>[2x]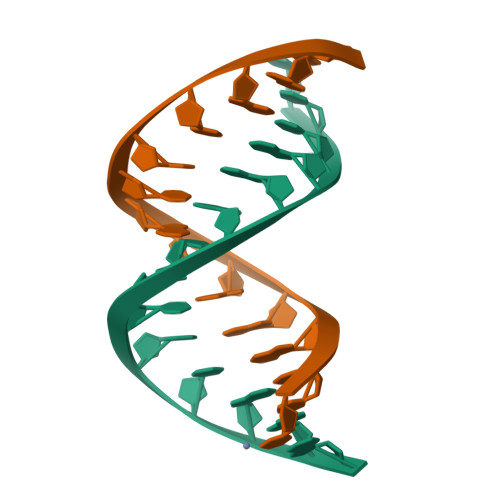CCCGGGTACCCGGG>[4x]METFTVKMGADSGLLQFEPANVTVHPGDTVKWVNNKLPPHNILFDCKQVPGASKELA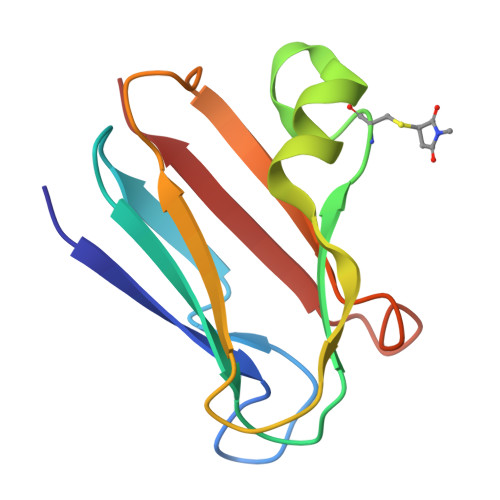DKLSHSQLMFSPGESYEITFSSDFPAGTYTYYCAPHRGAGMVGKITVEG NICOTINAMIDE-8-IODO-ADENINE-DINUCLEOTIDE | C21 H27 I N7 O14 P2 | 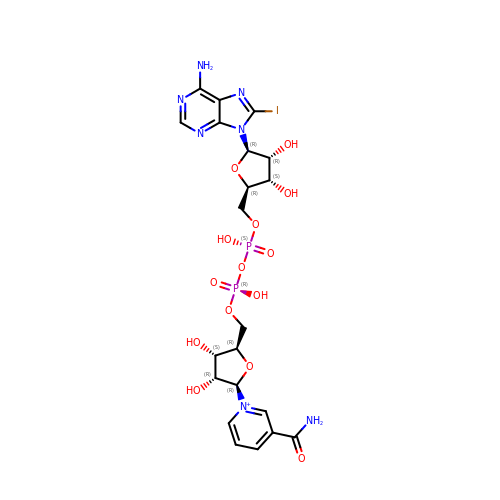UVGUXLRSEVQZMG-NAJQWHGHSA-O> MTLKALAQSLGITLKYLFSKPVTVPYPDAPVALKPRFHGRHVLTRHPNGLEKCIGCSLCAAACPAYAIYVEPAENDPENP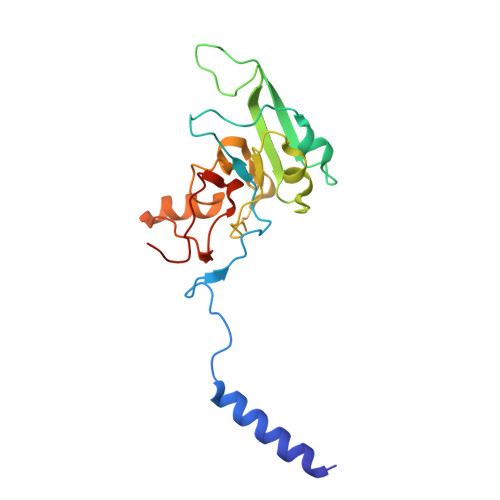VSAGERYAKVYEINMLRCIFCGLCEEACPTGAIVLGYDFEMADYEYSDLVYGKEDMLVDVVGTKPQRREAKRTGKPVKVGYVVPYVRPELEGFKAPTEGGKR>[6x]MFGYFYNSSFRRYATLMGDLFSNIQIKRQLESGDKFIRVPITYASKEHFMMKLNKWTSINSQEDVAKVETILPRINLHLVDFSYNAPFKTNILNQNLLQKGATSVVSQYNPSPIKMIYELSIFTRYEDDMFQIVEQILPYFQPHFNTTM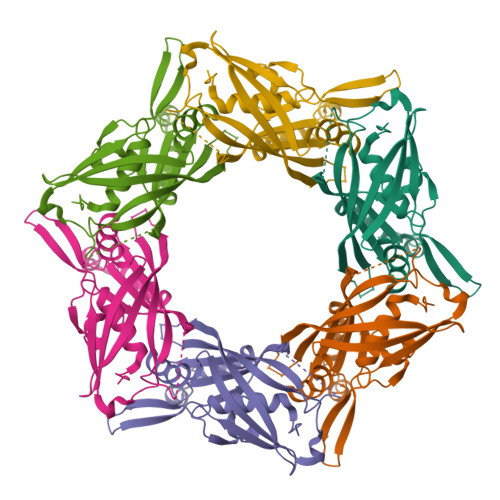YEQFGNDIPFKRDIKIVLMSAAIDEAIDGDNLSRRRIEWSLTFEVNGWMYPPVDDAEGLIRTTYTDFHANTRDLPDGEGVFESVDSEVVPRDIDPEDWDGTVKQTFTSNVNRPTPPEPPGPRT> PYV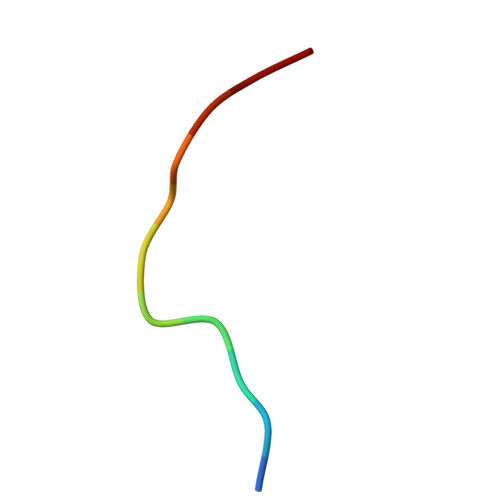PVHFAASV> MFADVETTCCARRTLTTIDEVPGMADETALLDWLGTMREKQPVWQDRYGVWHVFRHADVQTVLRDTATFSSDPTRVIEGASPTPGAIHEIDPPEHRALRKVVSSAFTPRTISDLEPRIRDVTRSLLADAGESFDLVDVLAFPLPVTIVAELLGLPPMDHEQFGDWSGALVDIQMDDPTDPALAERIADVLNPLTAYLKARCAERRADPGDDLISRLVLAEVDGRALDDEEAANFSTALLLAGHITTTVLLGNIVRTLDEHPAHWDAAAEDPGRIPAIVEEVLRYRPPFPQMQRTTTKATEVAGVPIPADVMVNTWVLSANRDSDAHDDPDRFDPSRKSGGA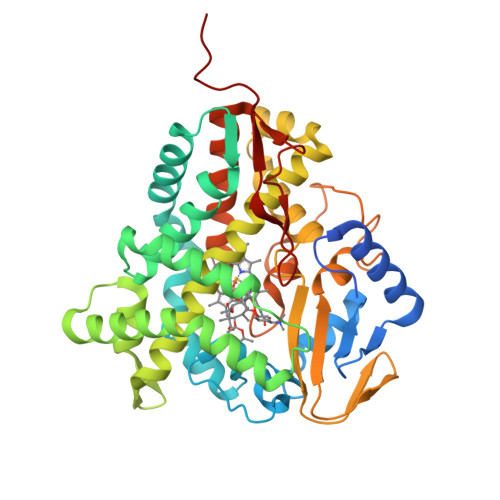AQLSFGHGVHFCLGAPLARLENRVALEEIIARFGRLTVDRDDERLRHFEQIVLGTRHLPVLAGSSPRQSA> GAMIESSTTIQVISAGLPRTGTKSLKNALEIIYHKPCYHMFEIIFNKQSDIIKWQNLIHDSHMITTPPPLTTKTIAIYDKLKELLDGYIATTDLPTCGFYKDLMNIYPNAKVLLTIRDKYDWLHSLRKVVLPKSNDPWKLKIEEGDKVLGLNSDFYKLSEDSLKFAFQKDDLNFDDDQVLLECYDEYNRLVQETVPSDRLLVLRLGDGWEPLCKFLNVEIPNGIDYPCVNSHHQMTQLTEQLIKYKSLDAIIHMFPD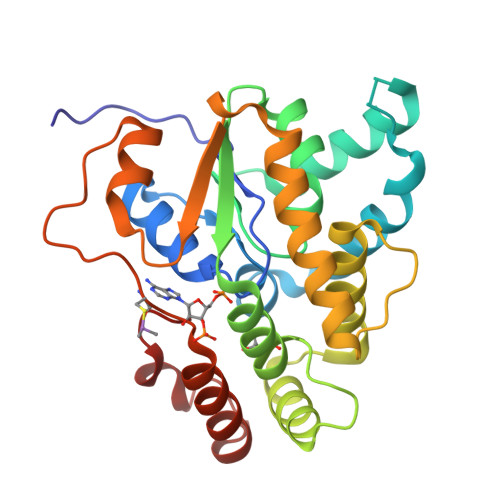LI>[2x]GTSMETFDPTELPELLKLYYRRLFPYSQYYRWLNYGGVIKNYFQHREFSFTLKDDIYIRYQSFNNQSDLEKEMQAANPYKIDIGAVYSHRPNQHNTVKLGAFQAQEKELVFDIDMTDYDDVRRCCSSADICPKCWTLMTMAIRIIDRALKEDFGFKHRLWVYSGRRGVHCWVCDESVRKLSSAVRSGIVEYLSLVKGGQDVKK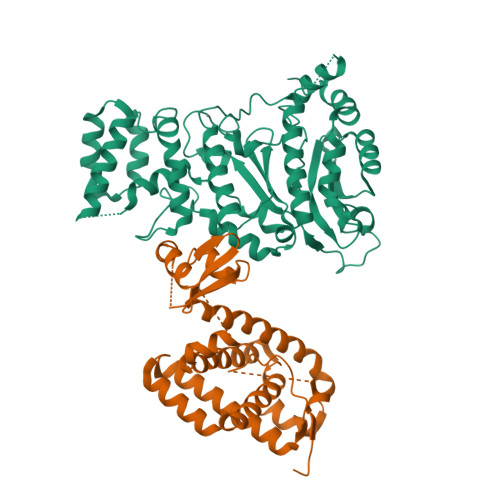KVHLSEKIHPFIRKSINIIKKYFEEYALVNQDILENKESWDKILALVPETIHDELQQSFQKSHNSLQRWEHLKKVASRYQNNIKNDKYGPWLEWEIMLQYCFPRLDINVSKGINHLLKSPFSVHPKTGRISVPIDLQKVDQFDPFTVPTISFICRELDAISTNEEEKEENEAESDVKHRTRDYKKTSLAPYVKVFEHFLENLDKSRKGELLKKSDLQKDF;>MGYSEVNLSKLFAGCAVKSTGSTGSTGSTGSTGSNASYPHCLQFYLQPPSENISLIEFENLAIDRVKLLKSVENLGVSYVKGTEQYQSKLESELRKLKFSYRENLEDEYEPRRRDHISHFILRLAYCQSEELRRWFIQQEMDLLRFRFSILPKDKIQDFLKDSQLQFEAISDEEKTLREQEIVASSPSLSGLKLGFESIYKIPFADALDLFRGRKVYLEDGFAYVPLKDIVAIILNEFRAKLSKALALTARSLPAVQSDERLQPLLNHL[2x]> AFNNNPSSVGAYSSGTYRNLAQEMGKTNIQQKVNSTFDNMFGYNNTQQLYYPYTENGVYKAHYIKAINPDEGDDIRTEGQSWGMTAAVMLNKQEEFDNLWRFAKAYQKNPDNHPDAKKQGVYAWKLKLNQNGFVYKVDEGPAPNGEEYFAFALLNASARWGNSGEFNYYNDAITMLNTIKNKLMENQIIRFSPYIDNLTDPSYHIPAFYDYFANNVTNQADKNYWRQVATKSRTLLKNHFTKVSGSPHWNLPTFLSRLDGSPVIGYIFNGQANPGQWYEFDAWRVIMNVGLDAHLMGAQAWHKSAVNKALGFLSYAKTNNSKNCYE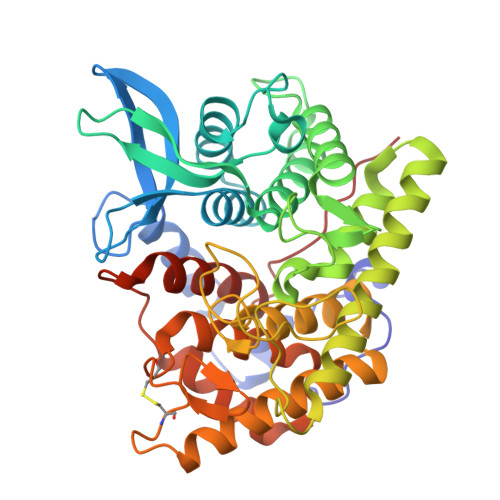QVYSYGGAQNRGCAGEGQKAANAVALLASTNAGQANEFFNEFWSLSQPTGDYRYYNGSLYMLAMLHVSGNFKFYNNTFN>SNAMSRAKKWVQYFLSHRHVTMELIHKIDEAHYDYKPTPTSMTAKQLATHMLFSFYNFANTAKHGDPSLFRQKIEEPETNLAKLAETYTEKTRQLIESMSDDDF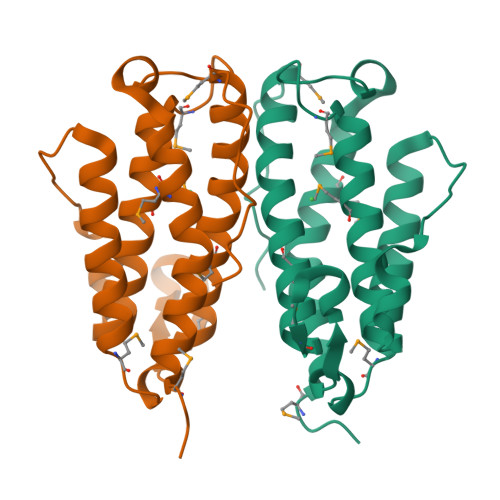DRTLDLTAIFGTQMSTAQFLQLAMDHEIHHKGQLFVYVRGMGHTDLPLFVKRG[4x]> LYCYE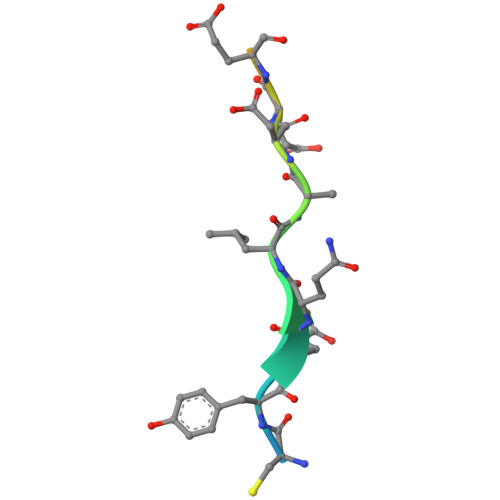QLNDEEEEEDEID(3S)-3-{[(5-BROMOPYRIDIN-3-YL)CARBONYL]AMINO}-4-OXOBUTANOIC ACID 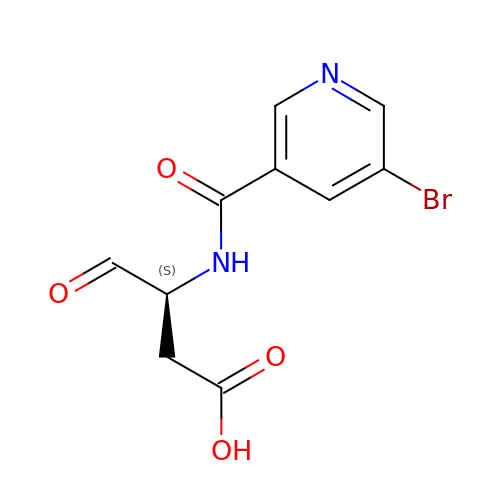| C10 H9 Br N2 O4 | FBMPVEGAIMRCBG-QMMMGPOBSA-N> MNYDI;> 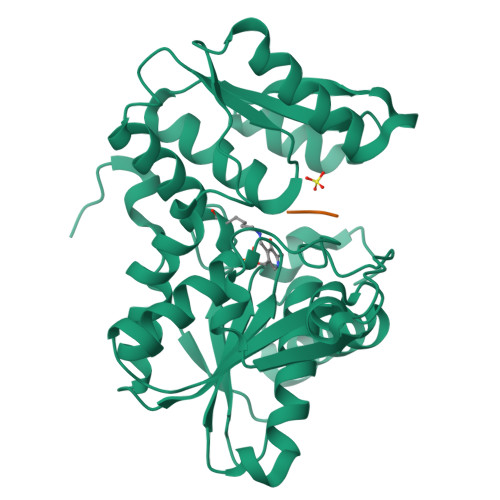MAIYADNSYSIGNTPLVRLKHFGHNGNVVVKIEGRNPSYSVKCRIGANMVWQAEKDGTLTKGKEIVDATSGNTGIALAYVAAARGYKITLTMPETMSLERKRLLCGLGVNLVLTEGAKGMKGAIAKAEEIVASDPSRYVMLKQFENPANPQIHRETTGPEIWKDTDGKVDVVVAGVGTGGSITGISRAIKLDFGKQITSVAVEPVESPVISQTLAGEEVKPGPHKIQGIGAGFIPKNLDLSIIDRVETVDSDTALATARRLMAEEGILAGISSGAAVAAADRLAKLPEFADKLIVVILPSASERYLSTALFEGIEG> AILNILEFPDPRLRTIAKPVEVVDDAVRQLIDDMFETMYEAPGIGLAATQVNVHKRIVVMDLSEDKSEPRVFINPEFEPLTEDMDQYQEGCLSVPGFYENVDRPQKVRIKALDRDGNPF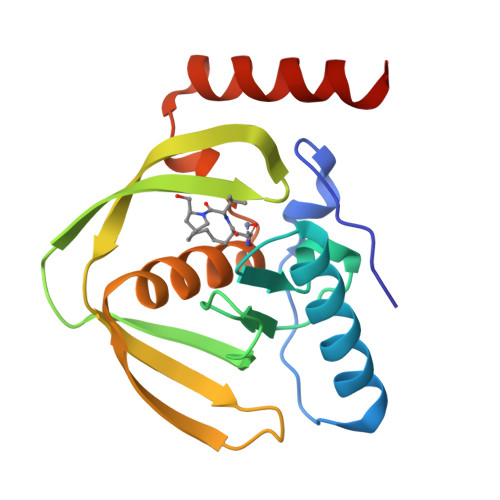EEVAEGLLAVCIQHECDHLNGKLFVDYLSTLKRDRIRKKLEKQHRQQA> APKAPADGLKMDKTKQPVVYNHSTHKAVKCGDCHHPVNGKEDY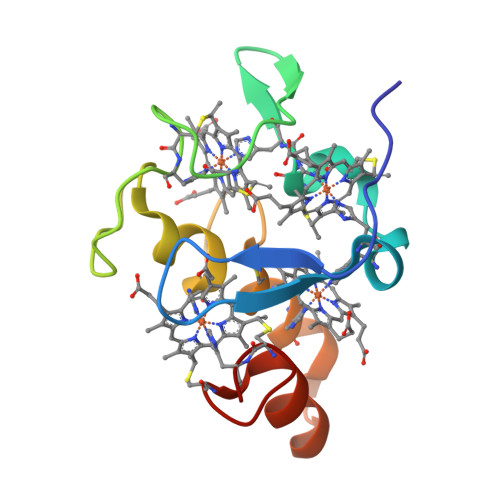QKCATAGCHDNMDKKDKSAKGYYHAMHDKGTKFKSCVGCHLETAGADAAKKKELTGCKGSKCHS~{N}-[4-[[5-fluoranyl-7-(2-methoxyethoxy)quinazolin-4-yl]amino]phenyl]-2-(4-propan-2-yl-1,2,3-triazol-1-yl)ethanamide 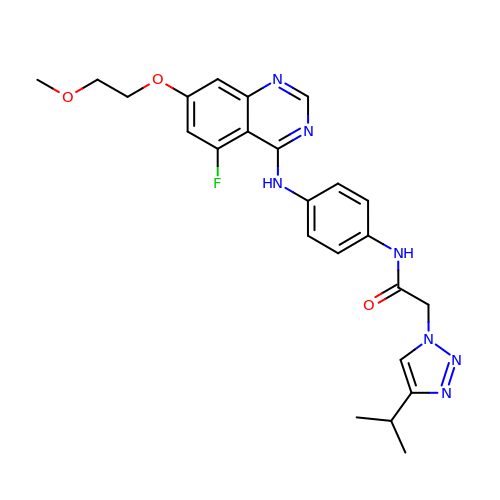| C24 H26 F N7 O3 | FLJOFQUXYAWOPE-UHFFFAOYSA-N pmcZinc (Zn)-dependent histone deacetylases (HDACs) are a family of 11 evolutionarily related hydrolases that catalyze the removal of acyl residues from histones, non-histone proteins, and polyamines. HDAC6 stands out among the 11 human isoforms, as being the only one that has two homologous tandem catalytic domains (CD1 and CD2). Furthermore, HDAC6 is mainly localized in the cytoplasm, and its main substrates are various non-histone proteins, such as α-tubulin, Foxp3, Hsp90, β-catenin, cortactin, and peroxiredoxins. By combining kinetics, X-ray crystallography, and mass spectrometry, we found that DFMO derivatives are slow-binding substrate analogs of HDAC6 that undergo an enzyme-catalyzed ring opening reaction, forming a tight and long-lived enzyme–inhibitor complex.

To gain further experimental insight into the mechanism of inhibition of HDAC6 by DFMOs, 1 was cocrystallized with zHDAC6-CD2. Surprisingly, the refined electron density of the bound ligand was not compatible with the inhibitor structure and suggested that a DFMO ring opening reaction had occurred. Several reaction mechanisms were hypothesized, and the resulting substructures were aligned with the experimental electron density map. In this procedure, a hydrazide moiety showed the best fit to the experimental density. In the crystal structure, the hydrazide NH2 group is positioned to share a sp3 lone pair with the metal cation, whereas simultaneously acting as a HB donor with both catalytic key residues His573 and His574. The position of the ZBG carbonyl oxygen atom suggests a HB with Tyr745 rather than a bond with the Zn ion, indicating hydrazide monodenticity. The phenyl substructure directly bound to the ZBG is buried in the crevice made by Phe583 and Phe643, where aromatic rings are interacting through a three-body π–π interaction, whereas the C-H⋯X HB is formed with the methylene substructure and the key residue Ser531 (12, 13, 18). A weak π-alkyl bond is established between triazole and Leu712, whereas the phenyl substructure of the cap interacts with His462 and Pro464. Finally, the apical 2-aminoimidazoline is bound to Asp460 through multiple HBs. When incubated with zHDAC6-CD2, 1 is converted into 2 first and 3 thereafter. Taken together, these data indicate that the complex with 1 itself and the hydrazide 3 observed in the crystal structure are unlikely to be the long-lived enzyme–inhibitor complex detected kinetically.

>[2x]GSNAGGSSPITGLVYDQRMMLHHNMWDSHHPELPQRISRIFSRHEELRLLSRCHRIPARLATEEELALCHSSKHISIIKSSEHMKPRDLNRLGDEYNSIFISNESYTCALLAAGSCFNSAQAILTGQVRNAVAIVRPPGHHAEKDTACGFCFFNTAALTARYAQSITRESLRVLIVDWDVHHGNGTQHIFEEDDSVLYISLHRYEDGAFFPNSEDANYDKVGLGKGRGYNVNIPWNGGKMGDPEYMAAFHHLVMPIAREFAPELVLVSAGFDAARGDPLGGFQVTPEGYAHLTHQLMSLAAGRVLIILEGGYNLTSISESMSMCTSMLLGDSPPSLDHLTPLKTSATVSINNVLRAHAPFWSSLR> QIGELKTTVGNSTIKVNDEVQVGSAFEAILGIEGLNGDTEVYSAEYLFEYNAEAFILNEITSF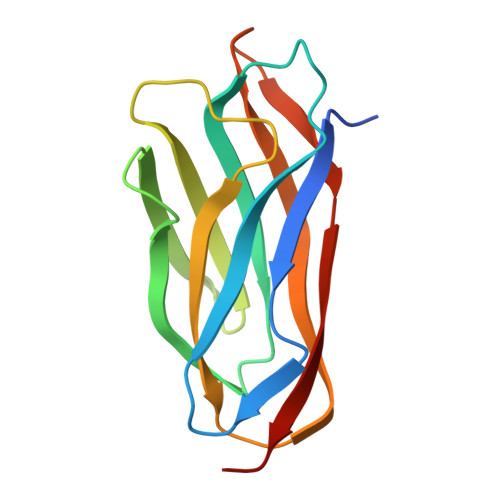NDSLFVKSKEVEPGKVRILVASLGNEIEKDSDLVKVNLTPKISSELEVLGLTTALVGAGDGNTHDLELSSKEVKINEEAS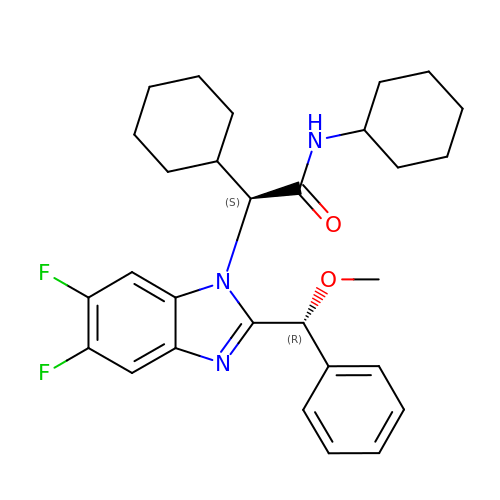(2S)-N,2-dicyclohexyl-2-{5,6-difluoro-2-[(R)-methoxy(phenyl)methyl]-1H-benzimidazol-1-yl}acetamide | C29 H35 F2 N3 O2 | URGAGGFDWSHABX-RRPNLBNLSA-N>MQIPASEQETLVRPKPLLLKLLKSVGAQKDTYTMKEVLFYLGQYIMTKRLYDEKQQHIVY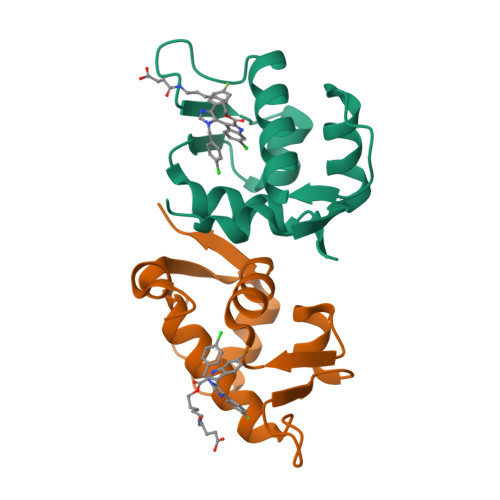CSNDLLGDLFGVPSFSVKEHRKIYTMIYRNLVVVNQQESSDSGTSVSEN[4x]The lipid-enveloped bacteriophages of the Cystoviridae family infect Gram-negative bacteria, mainly plant-pathogenic Pseudomonas species and share similarities with the members of the Reoviridae family, including bluetongue virus and rotavirus. Their genome of ∼14 kb consists of three dsRNA segments small (S), medium (M) and large (L), which are sequentially encapsidated as ssRNA precursors into the icosahedrally symmetric procapsid by the packaging NTPase P4 (15–23). P4 is a protein of ∼35 kDa, which can assemble into a hexameric ring. NTP-binding sites are located on the external perimeter of the ring at the interfaces between adjacent subunits, whereas the nucleic acid binding sites are found in the central channel. P4 proteins are the only known RNA-specific helicases belonging to helicase Superfamily 4 (SF4).

The ɸ6 P4 was crystallised with ADP-Mg2+ bound in the nucleotide binding site, whereas P4 from ɸ8 and ɸ13 were crystallized in their apo form. As for ɸ12 P4, and other hexameric NTPases, the nucleotide binding sites in ɸ6 P4 are located at the interfaces between neighbouring subunits. The ADP phosphate groups are bound via the conserved Walker A (H1) motif residues (K132, S133); a conserved glutamate E150 (H1a) is positioned to catalyse the nucleophilic attack on the γ-phosphate, whereas D187, a conserved aspartate in the Walker B motif (H2), co-ordinates the magnesium ion. A sensor motif detecting the presence or absence of the γ-phosphate of NTP and modulating allosteric transitions of the RNA binding loop L2 in response to ATP binding and hydrolysis was identified in P4 from ɸ12 (N234). The equivalent residue in ɸ6 P4, N232, is positioned to contact the γ-phosphate of the NTP and might fulfil the same role. In ɸ6 P4, a much looser stacking of the nucleotide base is observed, with only one side chain (F275) stabilizing the adenine ring. In all P4 structures, the N-terminal domain covers the apical part of the hexamer, and in ɸ12 P4, an N-terminal domain α-helix projects from one subunit to the adjacent one, giving the hexamer a more rounded appearance. ɸ6 P4 lacks such a helix and might stabilize the hexamer by strengthening subunit interfaces with nucleotides. ɸ6 P4 is the only P4 that needs nucleotides and divalent cations to form hexamers. The structures of P4 from ɸ6 and ɸ13 show ordered L1 loops, which line the central channel and contact the L2 loops. The L2 loops are found with lysine residues (K239 and K265, respectively) projecting towards the centre of the channel, in the same position as K241 in ɸ12, suggesting a conserved mechanism for binding and translocating RNA. In P4 from ɸ6, ɸ12 and ɸ13, the arginine fingers are pointing towards the catalytic sites, making the subunits competent and primed for hydrolysis.

>[12x]MPIVVTQAHIDRVGIAADLLDASPVSLQVLGRPTAINTVVIKTYIAAVMELASKQGGSLAGVDIRPSVLLKDTAIFTKPKAKSADVESDVDVLDTGIYSVPGLARKPVTHRWPSEGIYSGVTALMGATGSGKSITLNEKLRPDVLIRWGEVAEAYDELDTAVHISTLDEMLIVCIGLGALGFNVAVDSVRPLLFRLKGAASAGGIVAVFYSLLTDISNLFTQYDCSVVMVVNPMVDAEKIEYVFGQVMASTVGAILCADGNVSRTMFRTNKGRIFNGAAPLAADTHMPSMDRPTSMKALDHTSIASVAP>[3x]MSLSYVHTEIQNDALYITLD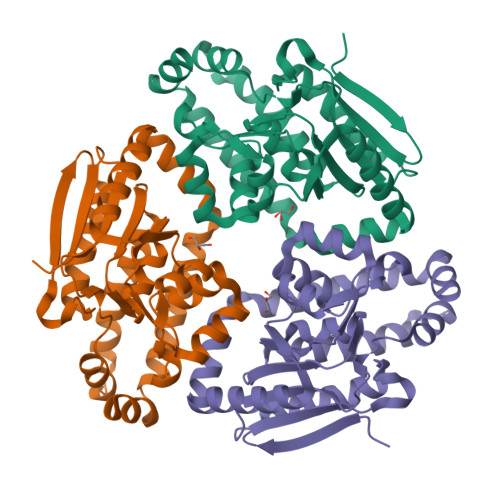YPEKKNGLDAELGTSLLEAIRAGNNETSIHSIILQSKHRAYFSSGPRLEDLLICASDQSDVRLREVLHVLNHCVLEIFTSPKVTVALINGYAYGGGFNMMLACDRRIALRRAKFLENFHKMGISPDLGASYFLPRIIGYEQTMNLLLEGKLFTSEEALRLGLIQEICENKQELQERVKNYLKAVSEGYVPAIAATKKLLKGKAAEELKQQLEQETEELVALFKQTEIKKRLEALVEGHHHHHH> GPLGSEAHLYMQVQIVAEDQFCGHQGNDMYDEEKVKYTVFKVLK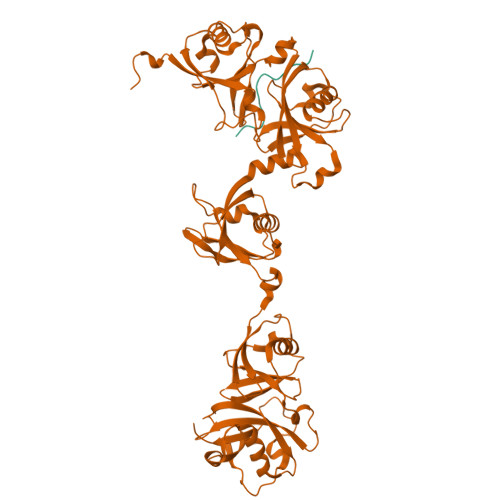NSSLAEFVQSLSQTMGFPQDQIRLWPMQARSNGTKRPAMLDNEADGNKTMIELSDNENPWTIFLETVDPELAASGATLPKFDKDHDVMLFLKMYDPKTRSLNYCGHIYTPISCKIRDLLPVMCDRAGFIQDTSLILYEEVKPNLTERIQDYDVSLDKALDELMDGDIIVFQKDDPENDNSELPTAKEYFRDLYHRVDVIFCDKTIPNDPGFVVTLSNRMNYFQVAKTVAQRLNTDPMLLQFFKSQGYRDGPGNPLRHNYEGTLRDLLQFFKPRQPKKLYYQQLKMKITDFENRRSFKCIWLNSQFREEEITLYPDKHGCVRDLLEECKKAVELGEKASGKLRLLEIVSYKIIGVHQEDELLECLSPATSRTFRIEEIPLDQVDIDKENEMLVTVAHFHKEVFGTFGIPFLLRIHQGEHFREVMKRIQSLLDIQEKEFEKFKFAIVMMGRHQYINEDEYEVNLKDFEPQPGNMSHPRPWLGLDHFNKAPKRSRYTYLEKAIKIHN;> SGPRGPRKCARKTRHAETSGA>[5x]MNHKVHMDVGTIIGIIAAF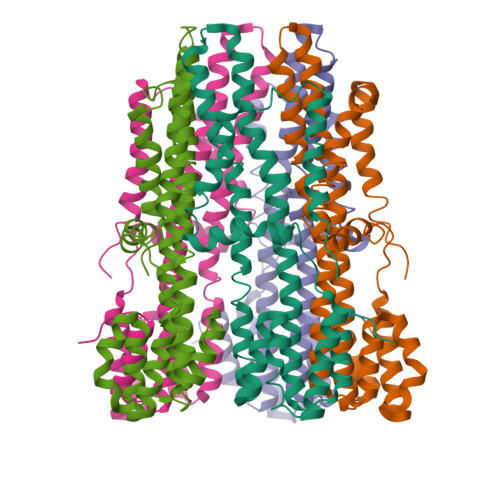LLILISILIGGSITAFINVPSIFIVVGGGMAAAMGAFPLKDFIRGVLAIKKAFLWKPPDLNDVIETIGEIASKVRKEGILALEGDIELYYQKDPLLGDMIRMLVDGIDINDIKATAEMALAQLDEKMSTEVAVWEKLADLFPAFGMIGTLIGLIQMLRNLNDPSALGPGMAVALITTLYGAILANAFAIPVANKLKKAKDMEVLVKTIYIEAIEKIQKGENPNVVKQEAAIMLGVELPEEVHHHHHH> MHHHHHHMKSIDEQSLHNARRLFESGDIDRIEVGTTAGLQQIHRYLFGGLYDFAGQIREDNISKGGFRFA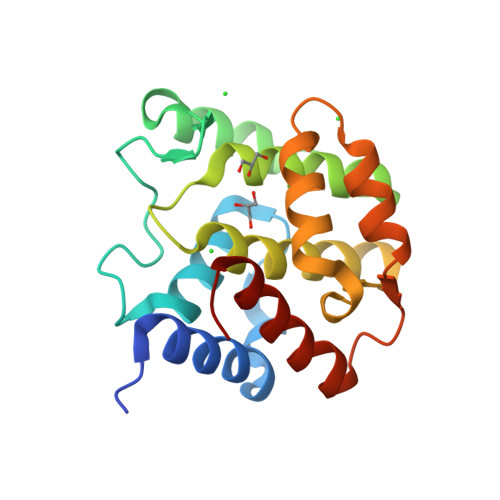NAMYLKEALVKIEQMPERTFEEIIAKYVEMNIAHPFLEGNGRSTRIWLDLVLKKNLKKVVNWQNVSKTLYLQAMERSPVNDLRLRFLLKDNLTDDVDNREIIFKGIEQSFYYEGYEKG> GPLSRKGIIPEEYVLTRLAEDPAEPRYRTRERRVDGSGSGSGSAAGSGSGSGSGSGAAAEDLQDLGVRFLQPFVNLLSKGTYWWMNAFIKTAHKKPIDLRAIGKLPIAMRALTNYQRLCVAFDAQARKDTQSPQGARAIWRALCHAFGRRLILSSTFRILADLLGFAGPLCIFGIVDHLGKENHVFQPKTQFLGVYFVSSQEFLGNAYVLAVLLFLALLLQRTFLQASYYVAIETGINLRGAIQTKIYNKIMHLSTSNLSMGEMTAGQICNLVAIDTNQLMWFFFLCPNLWAMPVQIIVGVILLYYILGVSALIGAAVIILLAPVQYFVATKLSQAQRSTLEHSNERLKQTNEMLRGMKLLKLYAWESIFCSRVEVTRRKEMTSLRAFAVYTSISIFMNTAIPIAAVLITFVGHVSFFKESDLSPSVAFASLSLFHILVTPLFLLSSVVRSTVKALVSVQKLSEFLSSAEIREEQCAPREPAPQGQAGKYQAVPLKVVNRKRPAREEVRDLLGPLQRLAPSMDGDADNFCVQIIGGFFTWTPDGIPTLSNITIRIPRGQLTMIVGQVGCGKSSLLLATLGEMQKVSGAVF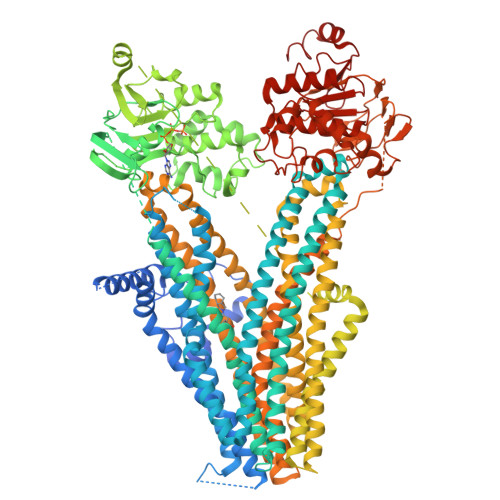WNSNLPDSEGEDPSSPERETAAGSDIRSRGPVAYASQKPWLLNATVEENITFESPFNKQRYKMVIEACSLQPDIDILPHGDQTQIGERGINLSGGQRQRISVARALYQQTNVVFLDDPFSALDVHLSDHLMQAGILELLRDDKRTVVLVTHKLQYLPHADWIIAMKDGTIQREGTLKDFQRSECQLFEHWKTLMNRQDQELEKETVMERKASEPSQGLPRAMSSRDGLLLDEEEEEEEAAESEEDDNLSSVLHQRAKIPWRACTKYLSSAGILLLSLLVFSQLLKHMVLVAIDYWLAKWTDSALVLSPAARNCSLSQECDLDQSVYAMVFTLLCSLGIVLCLVTSVTVEWTGLKVAKRLHRSLLNRIILAPMRFFETTPLGSILNRFSSDCNTIDQHIPSTLECLSRSTLLCVSALTVISYVTPVFLVALLPLAVVCYFIQKYFRVASRDLQQLDDTTQLPLLSHFAETVEGLTTIRAFRYEARFQQKLLEYTDSNNIASLFLTAANRWLEVRMEYIGACVVLIAAATSISNSLHRELSAGLVGLGLTYALMVSNYLNWMVRNLADMEIQLGAVKRIHALLKTEAESYEGLLAPSLIPKNWPDQGKIQIQNLSVRYDSSLKPVLKHVNALISPGQKIGICGRTGSGKSSFSLAFFRMVDMFEGRIIIDGIDIAKLPLHTLRSRLSIILQDPVLFSGTIRFNLDPEKKCSDSTLWEALEIAQLKLVVKALPGGLDAIITEGGENFSQGQRQLFCLARAFVRKTSIFIMDEATASIDMATENILQKVVMTAFADRTVVTIAHRVHTILSADLVMVLKRGAILEFDKPETLLSQKDSVFASFVRADK Ras suppressor protein 1 (Rsu1), a leucine-rich repeat (LRR)-containing protein conserved from human to worms, was recognized as a major FA component and is important for FA formation and cell motility. Among the IAC components, tripartite integrin-linked kinase (ILK) associates with another two key players PINCH and Parvin to form the ILK/PINCH/Parvin (IPP) complex, which acts as an essential platform to recruit many proteins for the FA formation and signaling and provide a linkage between FA and actin cytoskeleton. Here, we solved the crystal structures of the Rsu1/PINCH1 complex and found that Rsu1 strongly binds to PINCH1 through a large concave surface on its LRR solenoid. The cellular data supported the inhibitory effect of Rsu1 on the IPP complex. These results indicated that Rsu1, by interacting with PINCH1 and preventing PINCH1 from binding to actin, modulates actin dynamics at the FA and thereby regulates the stress fiber formation and cell adhesion dynamics.

On the other hand, the removal of the C-terminal region (aa.216–277) of Rsu1 (Rsu1ΔC) that does not belong to the LRR motif affected little to the complex formation of Rsu1 and PINCH1, suggesting that the LRR-region is sufficient for the Rsu1/PINCH1 interaction. We prepared the Rsu1/PINCH1 complex by combinatorial usage of the purified fragments that contains the elements necessary and sufficient for the Rsu1/PINCH1 interaction and successfully obtained the crystals of the Rsu1ΔC/PINCH1_LIM5C and Rsu1/PINCH1_LIM45C complexes. The complex structures of Rsu1ΔC/PINCH1_LIM5C with one crystal form at 1.65 Å resolution and Rsu1/PINCH1_LIM45C with two different crystal forms at 2.2 Å and 3.15 Å resolution respectively were determined by the molecular replacement method. Consistently, the deletion of C-cap results in the disruption of LRR9 in the Rsu1ΔC/PINCH1_LIM5C complex. In all three complex structures that we solved, the LIM5C fragment in PINCH1 and the LRRs in Rsu1 showed the essentially same conformation with the overall RMSD of ~0.3 Å. The large PINCH1-binding surface on Rsu1 extends from LRR2 to LRR9, in which 22 surface residues form hydrogen bonds, salt bridges, and hydrophobic interactions with PINCH1_LIM5C. These polar and hydrophobic interactions are interlaced with each other to provide the complementary binding required for the highly specific recognition between Rsu1 and PINCH1. Interestingly, although separately distributed at the interface, the polar interactions are well organized together by forming a hydrogen-bond network. In this network, two buried water molecules, conserved in both the Rsu1ΔC/PINCH1_LIM5C and Rsu1/PINCH1_LIM45C complex structures, critically coordinate three clusters of the polar interactions as highlighted in Figure 3D. Interestingly, the very C-terminal sequence (aa.308–325) in PINCH1 is indispensable for the binding of PINCH1 to Rsu1, as the LIM5 domain alone without this C-terminal sequence lost the Rsu1-binding ability.

> GAMGSMSKSLKKLVEESREKNQPEVDMSDRGISNMLDVNGLFTLSHITQLVLSHNKLTMVPPNIAELKNLEVLNFFNNQIEELPTQISSLQKLKHLNLGMNRLNTLPRGFGSLPALEVLDLTYNNLSENSLPGNFFYLTTLRALYLSDNDFEILPPDIGKLTKLQILSLRDNDLISLPKEIGELTQLKELHIQGNRLTVLPPELGNLDLTGQKQVFKAEN;> GPGSGDVCFHCNRVIEGDVVSALNKAWCVNCFACSTCNTKLTLKNKFVEFDMKPVCKKCYEKFPLELKKRLKKLAETLGRK> MTAFRQRPLRLGHRGAPLKAKENTLESFRLALEAGLDGVELDVWPTRDGVFAVRHDPDTPLGPVFQVDYADLKAQEPDLPRLEEVLALKEAFPQAVFNVELKSF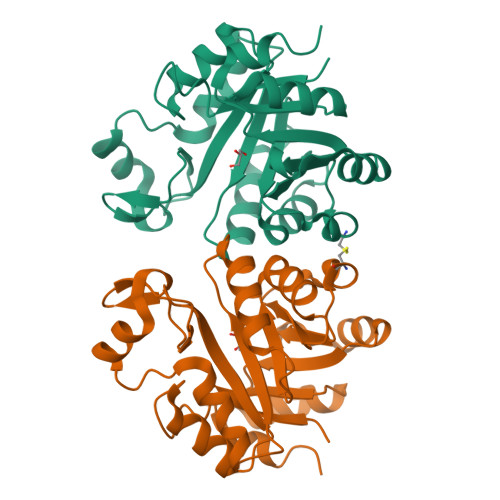PGLGEEAARRLAALLRGREGVWVSSFDPLALLALRKAAPGLPLGFLMAEDHSALLPCLGVEAVHPHHALVTEEAVAGWRKRGLFVVAWTVNEEGEARRLLALGLDGLIGDRPEVLLPLGG>GMETTVKIASDSSYAPFEFQNGQKKWVGIDVDIMQEVAKINDWKLEMSYPGFDAALQNLKAGQVDGIIAGMTITDERKETFDFSNPYYTSALTIATTKDSKLSDYSDLKGKAVGAKNGTAAQTWLQENQKKYGYTIKTYSDGVHM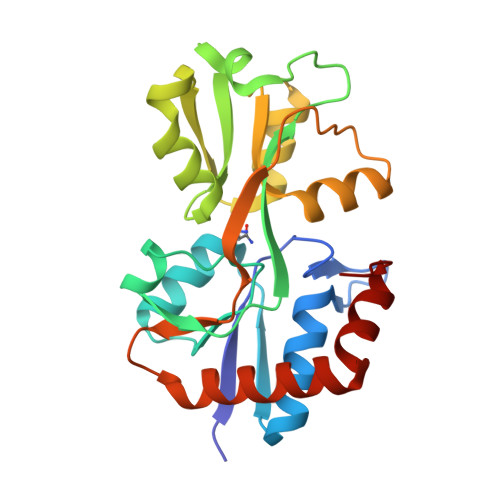FAALSSGNIAGAMDEVPVISYAMKQGQDLAMNFPSISLPGGYGFAVMKGKNSTLVDGFNKALAEMKSNGDYDKILKKYGITA[3x]(1R,2S)-2-(4-[bis(2-methylpropyl)amino]-3-{[(4-methylphenyl)carbamoyl]amino}phenyl)cyclopropane-1-carboxylic 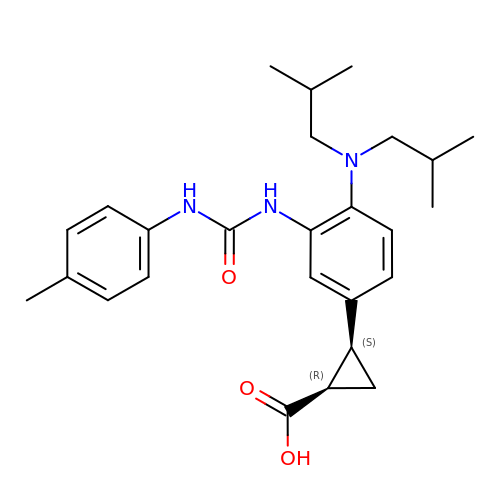acid | C26 H35 N3 O3 | VZYCPKLOYXSKAB-FGZHOGPDSA-N>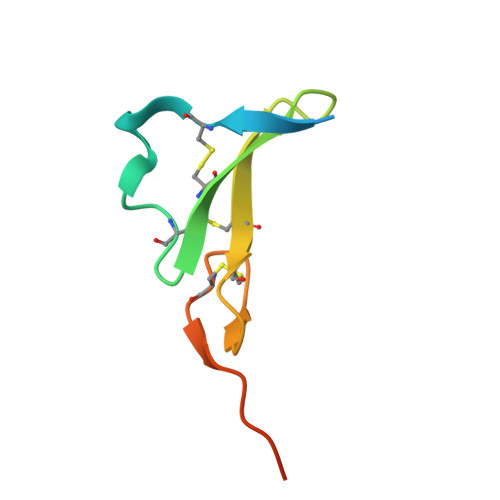 SDNPRVAQVSITKCSSDMNGYCLHGQCIYLVDMSQNYCRCEVGYTGVRCEHFFLTVHQPLSK>MFRLPTVMKQVRPVCRALAPHLTRAYAKDVKFGADARALMLQGVDLLADAVAVTMGPKGRTVIIEQSWGSPKVTKDGVTVAKSIDLKDKYKNIGAKLVQDVANNTNEEAGDGTTTATVLARAIAKEGFDTISKGANPVEIRRGVMMAVETVIKELKNLSKPVTTPEEIAQVATISANGDVEIGNIISNAMKKVGRKGVITVKDGKTLHDELEIIEGMKFDRGYISPYFINTAKGQKCEFQDAYLLLSEKKISSVQSIVPALEIANQHRKPLVIVAEDVDGEALSTLVLNRLKVGLQVVAVKAPGFGDNRKNQLRDMAVATGGTVFGDEAVGLALEDIQAHDFGKIGEVQITKDDTLLLKGGGSPAEVEKRAAEIVEQLENTTSDYEKEKLNERLAKLSDGVAVLKVGGTSDVEVNEKKDRVTDALNATRAAVEEGIVPGGGCALLRCIPSLDAIQTANADQKIGVEIIRRALRIPAMTIAKNAGVEGSLVVEKILQGSAELGY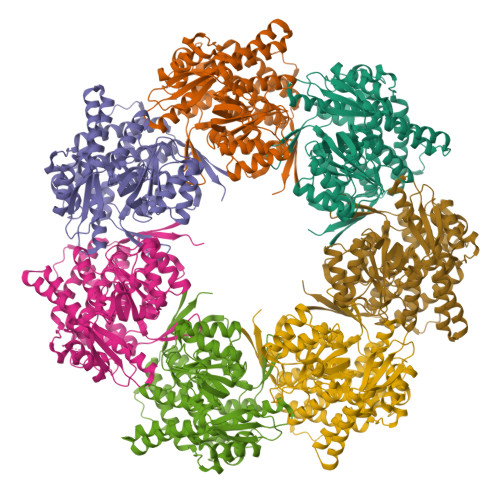DAMQGEYVNMVEKGIIDPTKVVRTALLDAAGVASLLSTAEAVVTEIPKEDIHMFRLPTGMGFLEHHHHHH[7x]The ferrous iron and 2-oxoglutarate (2OG)-dependent HIF prolyl hydroxylases (PHDs/EGLNs) catalyse trans-4-prolyl hydroxylations on HIFα subunits, thus promoting their binding to the von Hippel–Lindau protein (VHL), a targeting component of a ubiquitin E3 ligase, and signalling for HIFα degradation under normoxic conditions. The PHD-catalysed hydroxylations of HIF-1α/HIF-2α in higher animals occur in amino- and carboxy-terminal oxygen-dependent degradation domains (NODD and CODD). The three human PHDs exhibit different NODD/CODD selectivities, with PHD3 being substantially more selective for CODD than PHD1/2 (refs 16). Biophysical analyses employing crystallography and NMR reveal that the molecular basis of PHD isoform and variant selectivity involves enzyme–substrate interactions involving β2/β3 loop residues (that bind the LXXLAP motif) and helices α3 and α4, regions which display sequence variations between the PHD isoforms.

Analysis of a PHD2.N-oxalyl glycine (NOG).CODD complex structure led us to propose that certain erythrocytosis-associated PHD2 variants (P317R and R371H) would have altered substrate selectivities. R371H PHD2 retains >60% NODD activity and is equally active as wt PHD2 with CODD in endpoint assays; kinetic analyses show R371H is less efficient compared with wt PHD2 (for R371H, kcat/Km is reduced by ∼50% for NODD and CODD). Structures of the P317R, R371H and R396T variants with a clinically used inhibitor628 reveal similar overall folds to wt PHD2, that is, a modified double-stranded-β-helix (DSBH) core (β-strands I–VIII), supporting 2OG and His-X-Asp…His-mediated Fe(II) binding. The structures suggested that these variants probably manifest altered substrate binding, but do not explain how their differing NODD/CODD selectivities arise. Comparison of the structures rationalizes the selectivities of the clinically observed P317R, R371H and R396T variants. Arg371PHD2 (βVI-VII loop) apparently positions the Arg370PHD2 side chain in ODD binding: Arg370PHD2 interacts with both Asp395NODD (electrostatic) and Leu559CODD (hydrophobic); substitution of Arg370PHD2 with alanine did not affect CODD hydroxylation, but gave ∼35% reduction in NODD activity, demonstrating Arg370–Arg371 is more important in NODD than in CODD hydroxylation.

> GSHMASPNGQTKPLPALKLALEYIVPCMNKHGICVVDDFLGKETGQQIGDEVRALHDTGKFTDGQLVSQKSDSSKDIRGDKITWIEGKEPGCETIGLLMSSMDDLIRHCNGKLGSYKINGRTKAMVACYPGNGTGYVRHVDNPNGDGRCVTCIYYLNKDWDAKVSGGILRIFPEGKAQFADIEPKFDRLLFFWSDRHNPHEVQPAYATRYAITVWYFDADERARAKVKYLTGEKGVRVELNKPSDSVGKDVF>[4x]MSSDFATPPGLRHRQIAVRDTTLHVAEIGSGGTPVLLLHGWPEFWATWLPLMNRLHDQFHLIAPDLRGFGDSEKSAVPRSDVGANSHADDMAALLGALGLESVGVVGHDVGAYAAQALARRHPQLVDRLLFFNCPTASVGGAWVHHGHVNEVWYQSFQQLGLAEALVGTSRETCALYFRHFLEHWSHRKDAFEPAFELWIDNFMKPGNL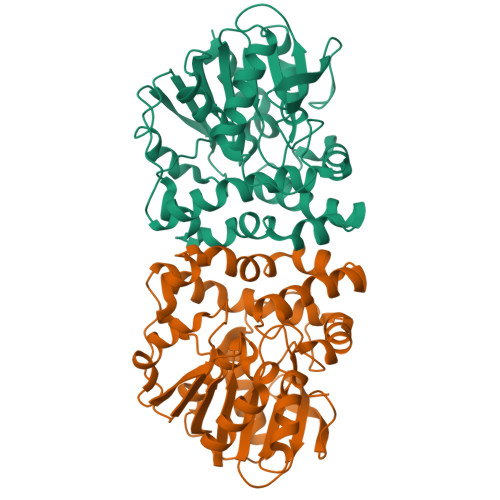RGGFDWYRSQNALRLAAIDGHPTPSVRIHQPTRVHWGRHDPILKSEWSAFVPEHFDDARISFCESAGHFVHVEAPDEAADVLAEFFGGR> ALVKEEIQAKEYLENLNKELAKRTNVETEAAWAYGSNITDENEKKKNEISAELAKFMKEVASDTTKFQWRSYQSEDLKRQFKALTKLGYAALPEDDYAELLDTLSAMESNFAKVKVCDYKDSTKCDLALDPEIEEVISKSRDHEELAYYWREFYDKAGTAVRSQFERYVELNTKAAKLNNFTSGAEAWLDEYEDDTFEQQLEDIFADIRPLYQQIHGYVRFRLRKHYGDAVVSETGPIPMHLLGNMWAQQWSEIADIVSPFPEKPLVDVSAEMEKQGYTPLKMFQMGDDFFTSMNLTKLPQDFWDKSIIEKPTDGRDLVCHASAWDFYLTDDVRIKQCTRVTQDQLFTVHHELGHIQYFLQYQHQPFVYRTGANPGFHEAVGDVLSLSVSTPKHLEKIGLLKDYVRDDEARINQLFLTALDKIVFLPFAFTMDKYRWSLFRGEVDKANWNCAFWKLRDEYSGIEPPVVRSEKDFDAPAKYHISADVEYLRYLVSFIIQFQFYKSACIKAGQYDPDNVELPLDNCDIYGSAAAGAAFHNMLSMGASKPWPDALEAFNGERIMSGKAIAEYFEPLRVWLEAENIKNNVHIGWTTSNKCVS

Human angiotensin I-converting enzyme (ACE; EC3.4.15.1) is a zinc metallopeptidase that plays a critical role in blood pressure regulation by catalysing the proteolysis of angiotensin I to the vasopressor angiotensin II. Because selenium compounds are known to exhibit better antioxidant behaviour than their sulfur analogues, we have recently reported the synthesis, characterization and antioxidant activity of a number of selenium analogues of the clinically used ACE inhibitor captopril. It was shown that selenium analogues of captopril (SeCap) not only inhibit ACE activity, but also can effectively scavenge peroxynitrite, a strong oxidant found in vivo. Here, we report for the first time, structural details on the binding of one of the potent SeCaps to tACE and AnCE, as elucidated by X-ray crystallography at 2.4 and 2.35 Å resolution, respectively. Captopril is one of the smallest ACE inhibitors and with both ACE and AnCE, key interactions of the selenium analogue's central carbonyl and proline carboxylate anchor the inhibitor in the cavernous S1′S2′-binding site of the enzyme.

AnCE is a single-domain protein, reported to have biochemical resemblance to C-domain ACE. The final structure contains a zinc ion, one inhibitor molecule, N-glycosylated carbohydrates at three potential binding sites (Asn53, Asn196, Asn311) and 201 water molecules. No noticeable conformational change is observed upon inhibitor binding. The topological arrangement of the final structure is consistent with previously determined structures of AnCE and AnCE in complex with captopril. One bound SeCap molecule was unambiguously fitted in the catalytic site of AnCE with the aid of a clearly observed electron-density map. The inhibitor SeCap molecule makes a direct interaction with the catalytic Zn2+ ion, displacing the water that is bound in the native enzyme (distance 2.7 Å), similar to the zinc coordination in AnCE–captopril. This interaction results in the formation of a zinc–selenolate complex. The carboxy-end of the proline moiety and the central carbonyl interact with the extended S1′S2′-binding site locking the inhibitor in position. The proline residue of SeCap makes important contacts with the S2′ subsite via two strong hydrogen bonds from two histidines (His497, 3.1 Å; His337, 2.5 Å). One oxygen atom of the proline carboxylate group interacts with Tyr504 (2.5 Å), Gln265 (2.9 Å) and Lys495 (2.9 Å) through hydrogen and ionic bonds.>MSRFIR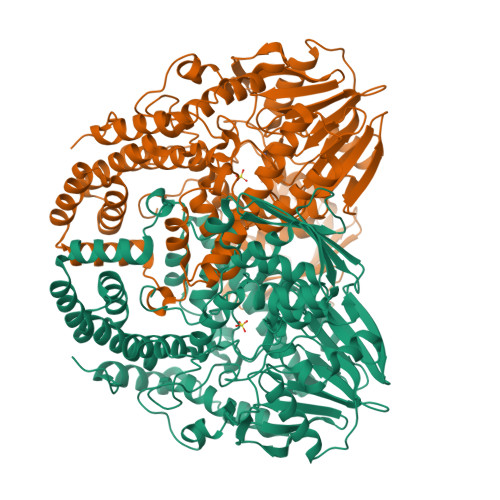ASQRRTLLATLIAATLAQPLLAAESLDSKPASAITAAKNAEVLKNLPFADREEFEAAKRGLIAPFSGQIKNAEGQVVWDMGAYQFLNDKDAADTVNPSLWRQAQLNNIAGLFEVMPKLYQVRGLDPANMTIIEGDSGLVLIDTLTTAETARAALDLYFQHRPKKPIVAVVYSHSHIDHFGGARGIIDEADVKAGKVKVFAPSGFMEHAVSENILAGTAMARRGQYQYGVMVPRGAQAQVDSGLGKTTATNATNTLVAPNVLIEKPYERHTVDGVELEFQLTLGSEAPSDMNIYLPQFKVLNTADNAPPAMHNLLTPRGAEVRDAKAWAGYIDASLEKYGDRTDVLIQQHNWPVWGGDKVRTYLADQRDMYAFLNNRALNLMNKGLTLHEIAAEVSKLPGELDRKWYLRSYYGALSTNLRAVYQRYLGFYDGNPANLDPFPPVEAGKRYVEAMGGADAVLKQMRAAIDKGDYRWAVQLGNHLVFADPANKDARALQADAMEQLGYQTENALWRNMYMTGAMELRHGVPTYDSRGKSEMGRALTPDMFFDLLAIRLDTDKAVGHDMTLNWVFEDLKQDIALTLRNGVLTQRVGSLNPKADVTVKLTKPTLDQIAARKLDLPTAIKQGTVKLDGDGKKLGEFFGLLDSFSPKFNIVELEHHHHHH[6x]>GAMPHDPSFTPTQLAARAAYLLRGNDLGTMTTAAPLLYPHMWSWDAAFVAIGLAPLSVERAVVELDTLLSAQWRNGMIPHIVFANGVDGYFPGPARWATATLADNAPRNRLTSGITQPPVHAIAVQRILEHARTRGRSTRAVAEAFLDRRWGDLMRWHRWLAECRDRNERGRITLYHGWESGMDNSPRWDSAYANVVPGKLPEYQRADNVIITDPSQRPSDGEYDRYLWLLEEMKAVRYDDERLPSVMSFQVEDVFFSAIFSVACQVLAEIGEDYKRPHADVKDLYLWAERFRAGVVETTDQRTGAARDFDVLAEKWLVTETAAQFAPLLCGGLPHDRERALLKLLEGPRFCGHPDLKYGLIPSTSPVSRDFRPREYWRGPVWPVLTWLFSWCFARRGWAERARLLRQEGLRQASDGSFAEYYEPFTGEPLGSMQQSWTAAAVLDWLG[2x]

A glucosylglycerate hydrolase (GgH) identified in M. hassiacum and found to be highly conserved among rapidly growing mycobacteria is likely to be responsible for the rapid mobilization of GG accumulated during nitrogen starvation by hydrolysing it to glucose and glycerate. The MhGgH monomer displays an (α/α)6-barrel domain typical of glycoside hydrolase family 63 (GH63), to which MhGgH belongs. While the active site of GH63 members acting on larger substrates is located in an open, solvent-accessible cleft, those of MhGgH and of MgH from T. thermophilus are covered by a cap domain (subdivided into A′- and B′-regions) with constrained access through a narrow negatively charged tunnel. The crystallographic structure of MhGgH revealed a homotetrameric architecture, which is compatible with the oligomeric organization of the enzyme in solution as assessed by SAXS.

Orthorhombic crystals belonging to space group P21212 that diffracted X-rays to beyond 1.7 Å resolution at a synchrotron source were obtained. The orthorhombic crystals contained two MhGgH molecules (here termed A and B) in the asymmetric unit, which were modelled from residues Pro2 to Gly446. In the orthorhombic crystals, the MhGgH molecules adopt a closed conformation concomitant with the presence of two ligands, a molecule of glycerol and a molecule of serine, which are components of the crystallization buffer, at the active site (MhGgH–Ser–GOL). The glycerol molecule occupies subsite −1 and serine is found at subsite +1 of the active site, inducing a closed state of MhGgH that renders them inaccessible to the solvent. The substrate-interacting residues in the complexes between MhGgH variants and GG are organized in a very similar way to that of MhGgH–Ser–GOL [r.m.s.d.s of 0.19 Å (D182A) and 0.22 Å (E419A) for 14 Cα pairs]. The serine and glycerol molecules present in the active site of the MhGgH–Ser–GOL structure partially mimic the substrate, with serine superposing nicely with the glycerate moiety and with glycerol establishing contacts with Asp43, a substrate placeholder that stabilizes the sugar moiety [Fig. 4(b)]. Taken together, these results suggest that the MhGgH–Ser–GOL and variant–GG complexes are likely to reflect the substrate-binding mode of GG to wild-type MhGgH. The two structures of MhGgH, apo MhGgH and MhGgH–Ser–GOL, corresponding to its open and closed conformations, reveal the structural modifications that occur upon substrate binding. In the closed conformation, this loop interacts with the segment Ser431–Ser435 (with polar interactions between the side chain of Asn23 and Gln433 and Ser435) that contains the substrate-interacting residue Gln434, which faces the active site and binds to the substrate. Substrate binding contributes to the formation of an additional helix in this cap (residues 206–209) that is absent in the open conformation.> SYSGPIVVDPVTRIEGHLRIEVEVENGKVKNAYSSSTLFRGLEIILKGRDPRDAQHFTQRTCGVCTYTHALASTRCVDNAVGVHIPKNATYIRNLVLGAQYLHDHIVHFYHLHALDFVDVTAALKADPAKAAKVASSISPRKTTAADLKAVQDKLKTFVESGQLGPFTNAYFLGGHPAYYLDPETNLIATAHYLEALRLQVKAARAMAVFGAKNPHTQFTVVGGVTCYDALTPQRIAEFEALWKETKAFVDEVYIPDLLVVAAAYKDWTQYGGTDNFITFGEFPKDEYDLNSRFFKPGVVFKRDFKNIKPFDKMQIEEHVRHSWYEGAEARHPWKGQTQPKYTDLHGDDRYSWMKAPRYMGEPMETGPLAQVLIAYSQGHPKVKAVTDAVLAKLGVGPEALFSTLGRTAARGIETAVIAEYVGVMLQEYKDNIAKGDNVICAPWEMPKQAEGVGFVNAPRGGLSHWIRI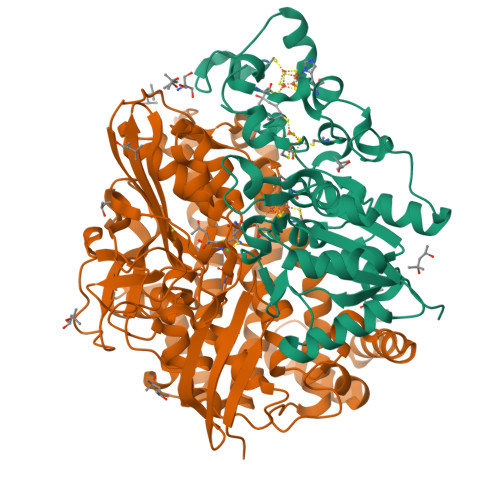EDGKIGNFQLVVPSTWTLGPRCDKNKLSPVEASLIGTPVADAKRPVEILRTVHSFDPCIACGVH;> GPRRPSVVYLHNAECTGCSESVLRAFEPYIDTLILDTLSLDYHETIMAAAGDAAEAALEQAVNSPHGFIAVVEGGIPTAANGIYGKVANHTMLDICSRILPKAQAVIAYGTCATFGGVQAAKPNPTGAKGVNDALKHLGVKAINIAGCPPNPYNLVGTIVYYLKNKAAPELDSLNRPTMFFGQTVHEQCPRLPHFDAGEFAPSFESEEARKGWCLYELGCKGPVTMNNCPKIKFNQTNWPVDAGHPCIGCSEPDFWDAMTPFYQN> MPVFHTRTIESILEPVAQQISHLVIMHEEGEVDGKAIPDLTAPVAAVQAAVSNLVRVGKETVQTTEDQILKRDMPPAFIKVENACTKLVQAAQMLQSDPYSVPARDYLIDGSRGILSGTSDLLLTFDEAEVRKIIRVCKGILEYLTVAEVVETMEDLVTYTKNLGPG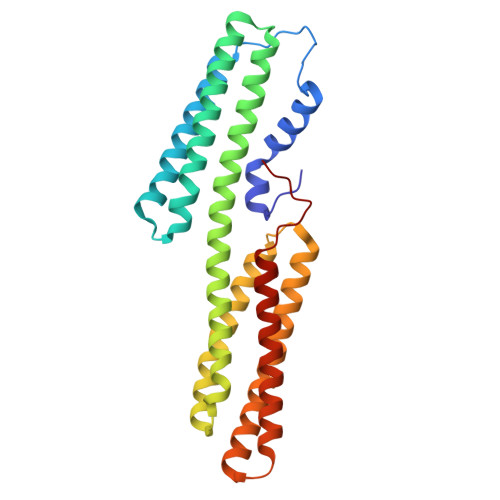MTKMAKMIDERQQELTHQEHRVMLVNSMNTVKELLPVLISAMKIFVTTKNSKNQGIEEALKNRNFTVEKMSAEINEIIRVLQLTSWDEDAW>[2x]MKVEEILEKALELVIPDEEEVRKGREAEEELRRRLDELGVEY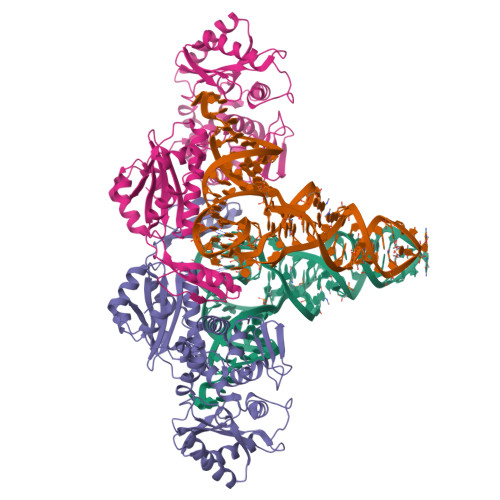VFVGSYARNTWLKGSLEIDVFLLFPEEFSKEELRERGLEIGKAVLDSYEIRYAEHPYVHGVVKGVEVDVVPCYKLKEPKNIKSAVDRTPFHHKWLEGRIKGKENEVRLLKGFLKANGIYGAEYKVRGFSGYLCELLIVFYGSFLETVKNARRWTRRTVIDVAKGEVRKGEEFFVVDPVDEKRNVAANLSLDNLARFVHLCREFMEAPSLGFFKPKHPLEIEPERLRKIVEERGTAVFAVKFRKPDIVDDNLYPQLERASRKIFEFLERENFMPLRSAFKASEEFCYLLFECQIKEISRVFRRMGPQFEDERNVKKFLSRNRAFRPFIENGRWWAFEMRKFTTPEEGVRSYASTHWHTLGKNVGESIREYFEIISGEKLFKEPVTAELCEMMGVKD> MEDTQA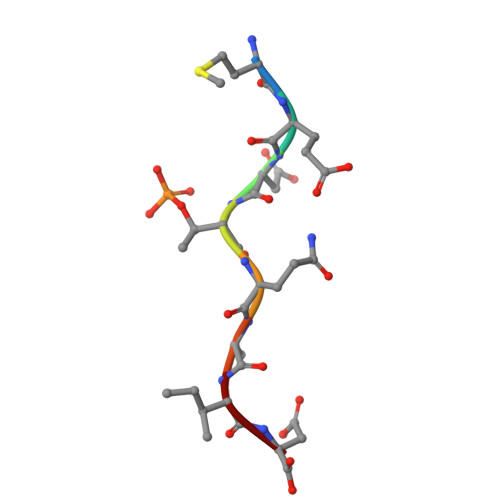ID3-fluoro-4-methylbenzenecarboximidamide | C8 H9 F N2 | 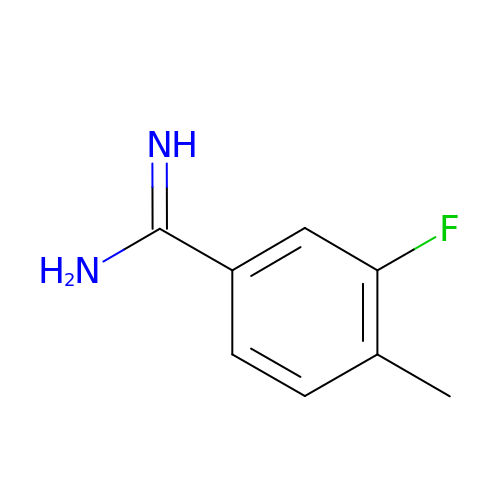PWQHQNWOXBOOTJ-UHFFFAOYSA-N>[5x]GSPGIPMLAVHFDKPGGPENLYVKEVAKPSPGEGEVLLKVAAS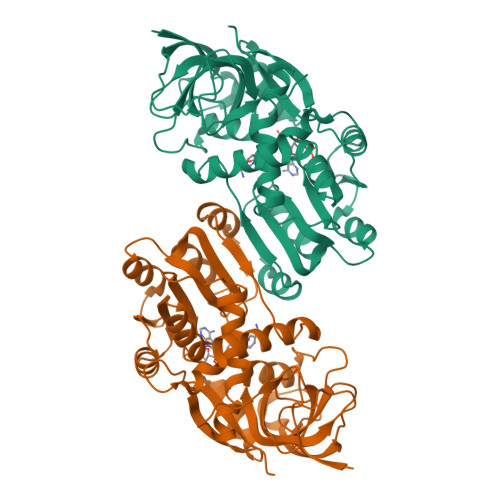ALNRADLMQRQGQYDPPPGASNILGLEASGHVAELGPGCQGHWKIGDTAMALLPGGGQAQYVTVPEGLLMPIPEGLTLTQAAAIPEAWLTAFQLLHLVGNVQAGDYVLIHAGLSGVGTAAIQLTRMAGAIPLVTAGSQKKLQMAEKLGAAAGFNYKKEDFSEATLKFTKGAGVNLILDCIGGSYWEKNVNCLALDGRWVLYGLMGGGDINGPLFSKLLFKRGSLITSLLRSRDNKYKQMLVNAFTEQILPHFSTEGPQRLLPVLDRIYPVTEIQEAHKYMEANKNIGKIVLELPQ>MTEHPAQQLYCTVVLWDLSRSAATVASLRAYLRDHAVDAYTTVPGLRQKTWISSTGPEGEQWGAVYLWDSPEAAYGRPPGVSKVVELIGYRPTERRYYSVEAATEGPAAAAAPFGKGLGLAFDPASPEPLTRPQEFVPPGADAFIP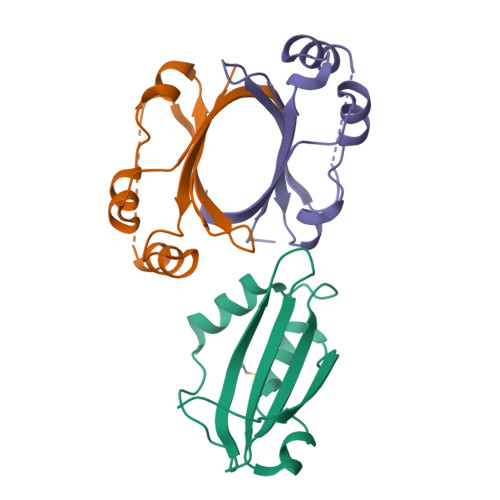SRPPA[3x]> MAHHHHHHDDKSVCDSDNKEYMGIEVYVEATLDEPLRQTTCESKIHKYGASVSNGGLNISV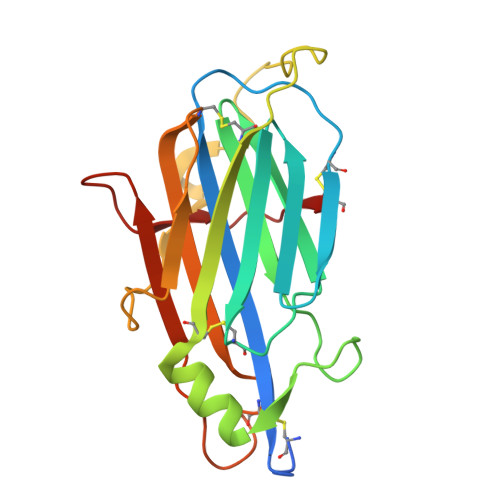DLLNCFLNFHTVGVYTNRDTVYAKFASLDPWTTEPINSMTHDDLVKLTEECIVDIYLKCEVDKTKDFMKTNGNRLKPRDFKTVPPSNVGSMIELQSDYCVNDVTTYVKIYDECGNIKQHSIPTLRDYFTTKNGQPRKILKKKFDNC>SPDKLKKVLDKLRLKRKDISEAAETVNKVVERLLRRMQKRESEFKGVEQLNTGSYYEHVKISAPNEFDVMFKLE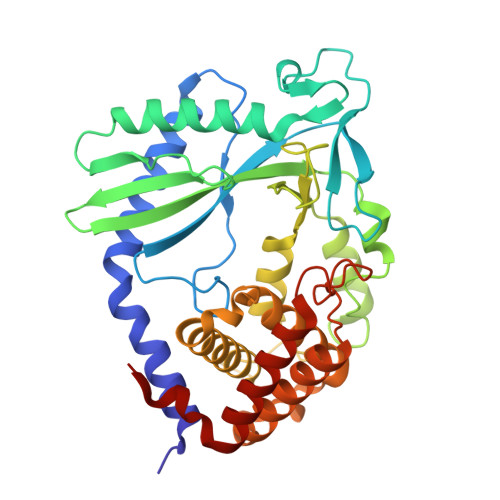VPRIELQEYYETGAFYLVKFKRIPRGNPLSHFLEGEVLSATKMLSKFRKIIKEEVKEIKDIDVSVEKEKPGSPAVTLLIRNPEEISVDIILALESKGSWPISTKEGLPIQGWLGTKVRTNLRREPFYLVPKNAKDGNSFQGETWRLSFSHTEKYILNNHGIEKTCCESSGAKCCRKECLKLMKYLLEQLKKEFQELDAFCSYHVKTAIFHMWTQDPQDSQWDPRNLSSCFDKLLAFFLECLRTEKLDHYFIPKFNLFSQELIDRKSKEFLSKKIEYERNNGFPIFDKL[4x]> GHMSGSNTEEEIRMELSPDLISACLALEKYLDNPNALTERELKVAYTTVLQEWLRLACRSDAHPELVRRHLVTF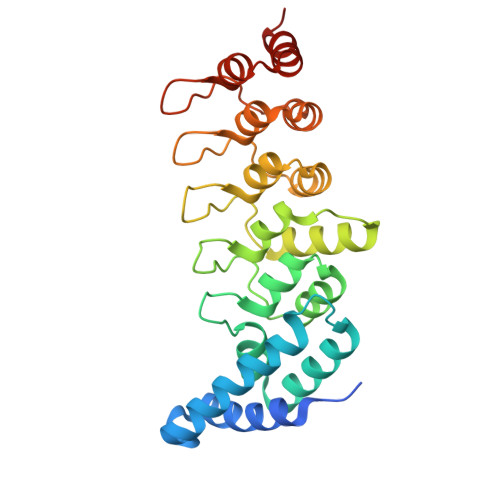RAMSARLLDYVVNIADSNGNTALHYSVSHANFPVVQQLLDSGVCKVDKQNRAGYSPIMLTALATLKTQDDIETVLQLFRLGNINAKASQAGQTALMLAVSHGRVDVVKALLACEADVNVQDDDGSTALMCACEHGHKEIAGLLLAVPSCDISLTDRDGSTALMVALDAGQSEIASMLYSRMNIK> MVELTEIKD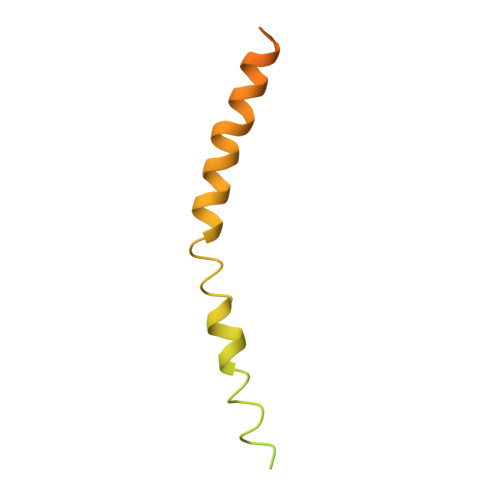DVVQLDEPQFSRNQAIVEEKASATNNDVVDDEDDSDSDFEDEFDENETLLDRIVALKDIVPPGKRQTISNFFGFTSSFVRNAFTKSGNLAWTLTTTALLLGVPLSLSILAEQQLIEMEKTFDLQSDANNILAQGEKDAAATANGSPGHHHHHHHHHH> XTEAA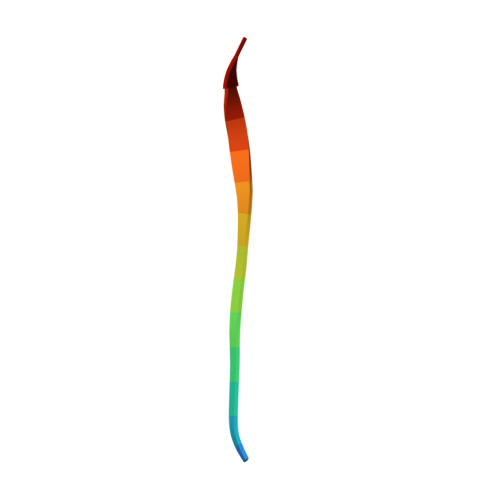AGMGGVMTGR[(2~{R})-1-hexadecanoyloxy-3-[oxidanyl-[2-(trimethyl-$l^{4}-azanyl)ethoxy]phosphoryl]oxy-propan-2-yl] (5~{Z},8~{Z},11~{Z},14~{Z})-icosa-5,8,11,14-tetraenoate | C44 H81 N O8 P | 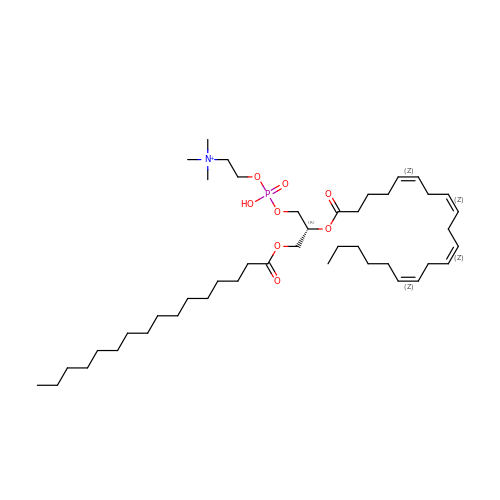IIZPXYDJLKNOIY-JXPKJXOSSA-O Siphophage T1 is representative of the T series of model Escherichia coli phages, which has been observed to infect not only sensitive strains of E. coli but also some strains of Shigella dysenteriae. Siphophages possess a long, flexible, and non-contractile tail that plays a crucial role in host recognition, cell envelope penetration, and DNA injection. Connected to the head through a connector complex, the tail of a siphophage consists of three main components: a tail tube, a tape measure protein (TMP), and a distal tip. Using cryo-EM, we resolved the three-dimensional (3D) structures of the icosahedral head, head–tail complex and the tail tip of a laboratory-adapted fiberless mature T1 at resolutions of 3.5 Å, 3.6 Å, and 4.3 Å, respectively.

The T1 head comprises 415 copies of the major capsid protein gp47, arranged into an icosahedron with a triangulation number of seven, decorated with 80 homologous trimers and 60 heterotrimers along the threefold and quasi-threefold axes of the icosahedron. The density maps enable us to build the atomic models for the MCP gp47 and CPs (gp48 and gp49), connector complex (portal gp52, adaptor gp45, stopper gp44, and tail terminator gp42), and TTP gp41.

>MTTKKFDEADKSNVEMYLIQAGVKQDAAATMGIWTAQELHRIKSQSYEEDYPVGSALRVFPVTTELSPTDKTFEYMTFDKVGTAQIIADYTDDLPLVDALGTSEFGKVFRLGNAYLISIDEIKAGQATGRPLSTRKASACQLAHDQLVNRLVFKGSAPHKIVSVFNHPNITKITSGKWIDVSTMKPETAEAELTQAIETIETITRGQHRATNILIPPSMRKVLAIRMPETTMSYLDYFKSQNSGIEIDSIAELEDIDGAGTKGVLVYEKNPMNMSIEIPEAFNMLPAQPKDLHFKVPCTSKCTGLTIYRPMTIVLITGV[7x];> MAYENLMLRPACPGNLSDTSTYNIDGACVAQGDIEFGSAVQVVGIVDGVKVVTALSDGGTPYGIAFRSQYEHLSGKILDGEVCNVVSHGRVWALTSLDEAPSLFSKLQFGSGGVVTGGSGYAGWTFAGGFVKHEDGYIIEVRVKQNAFIVPPPPPPVVLVESATITTDKESPQPNNVTIQCVANALPANATDKTGKWSIDATNIATVNPDSGLVTPVGGEVVGDFNITWTANDASKTTATIAYRVEAVPTPEVDV;>[6x]MAQINASYQRDMAIALPGMVADTSKYNIDGACVVNEGDVLVGAAVQVVQAQAVDGHKLVKALTTGTTPYGVAIRSHWQTVNAQNQMIYEDGGAINVMTSGRVWMLSKSTEAPTFGSAVKLDVDGQEKSDGTIETTWTYAGGWTKYKDIQLVEVQLHQL> MGDDLLLKLLELLVEQARVSAEFARRQGDEKMLEEVARKAEEVARKAEEIARKARKEGNLELALKALEILVR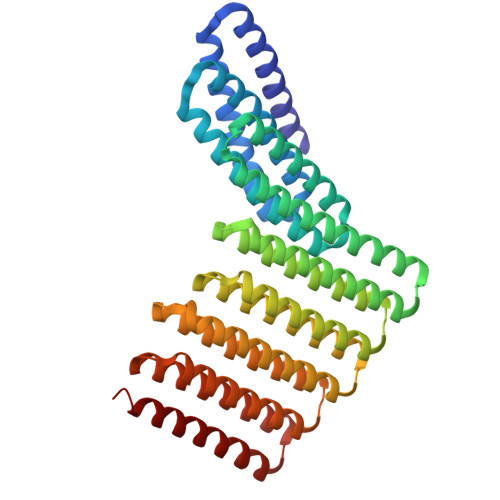AAHVLAEIARERGNEELQKKAHKLAKEALRQVIEIAIRAIQEGNLELAIIALHISVRIAEVLLETRPDDREEIREQQAIFELLIAALEAAIRLEKLKEEGAPPEQIERVAEHGLERLKEIAKEISKEVDSPESKRIAYKIVAAAAEFLLKILAEGGATPEQLERVTEHALEVLKEVAKELADSPESVREAVRLISKLTQEGLKQLKEIGAPPEQIERVAEHGLEVLKEIAKYGSKLTDSPELKRELYRIISETAKELLKILAEGGATPEQLERVTKHALEVLKEVAKELADSPESGLAALAAIASLAKLGLEQLKEIGAPPEQQRRVTKAGIEAVREIYRYGRKLY>[7x]MSEVQQLPIRAVGEYVILVSEPAQAGDEEVTESGLIIGKRVQGEVPELCVVHSVGPDV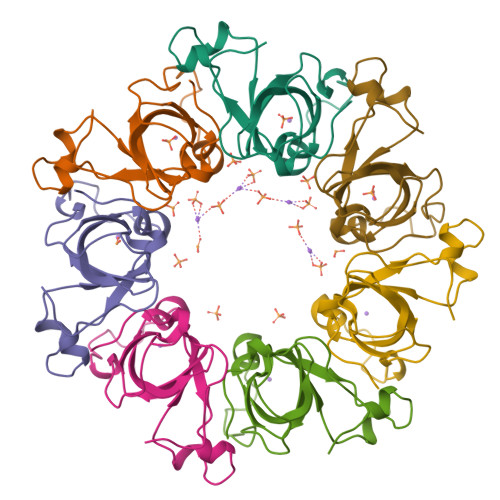PEGFCEVGDLTSLPVGQIRNVPHPFVALGLKQPKEIKQKFVTCHYKAIPCLYK2-BUTYL-6-HYDROXY-3-[2'-(1H-TETRAZOL-5-YL)-BIPHENYL-4-YLMETHYL]-3H-QUINAZOLIN-4-ONE | C26 H24 N6 O2 | 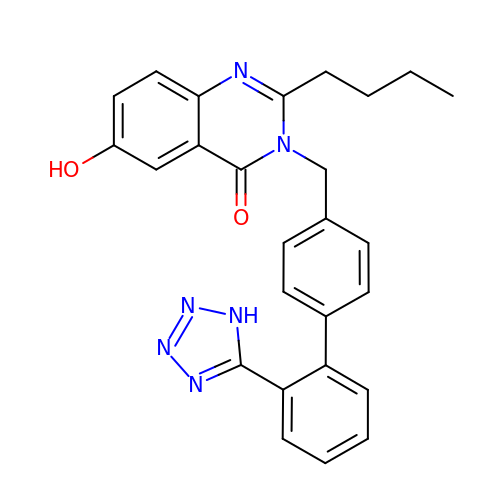UNVNHFHIKCWHHG-UHFFFAOYSA-N>[2x]GMSQTTVVNGVNVDQLMATIEQIKAKPEIAQFKFRATNQWMGGTHNQATIKDFYGACAEDDTRKPMVFDLDEPPVLLGENRGANPVEYLL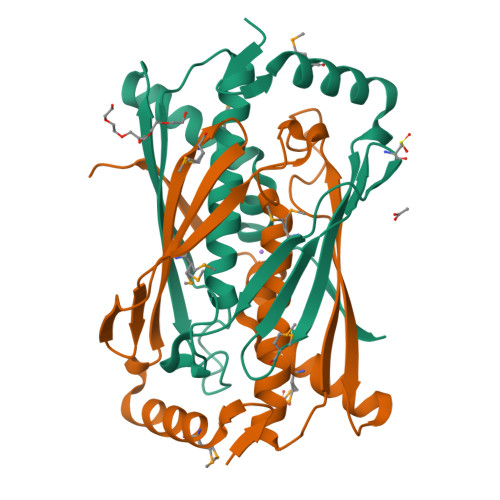VALSGCLTTSLVAHAAARGIALRGVKSRYEGDIDLRGFLGLSEEVPVGYREIRVFFSIDADLTDGQKEELIRMAQKYSPVYNTVAKPVPVAVLLDRG(1R,2S,4S,5'R,6R,7S,8R,9S,10R,12S,13S,16S,18S)-5',7,9,13-tetramethylspiro[5-oxapentacyclo[10.8.0.0^{2,9}.0^{4,8}.0^{13,18}]icosane-6,2'-oxane]-10,16-diol 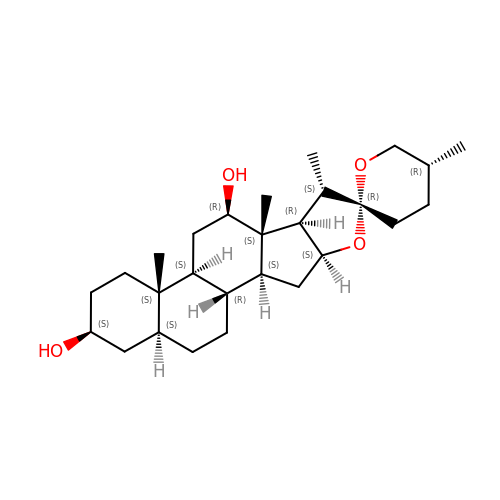| C27 H44 O4 | BQNMOLSYHYSCMS-TUUYSWIFSA-N> MRLERVLEEARAKGYPIEDNGLGNLWVVLPRERFKEEMAHYKAMGFNFLADIVGLDYLTYPDPRPERFAVVYELVSLPGW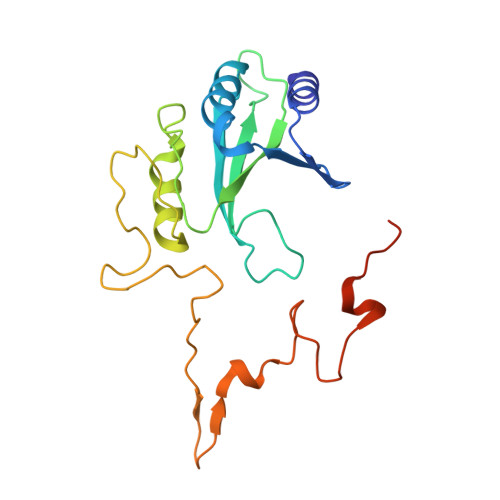KDGDGSRFFVRVYVPEEDPRLPTVTDLWGSANFLEREVYDLFGIVFEGHPDLRKILTPEDLEGHPLRKDYPLGETPTLFREGRYIIPAEFRAALTGKDPGLTFYKGGSRKGYRSLWADLKKAREVKG> SKLQATKTLAADVIMRSPVSWKQELTLDAGRSKGASENMLAIANGGLIGSVSK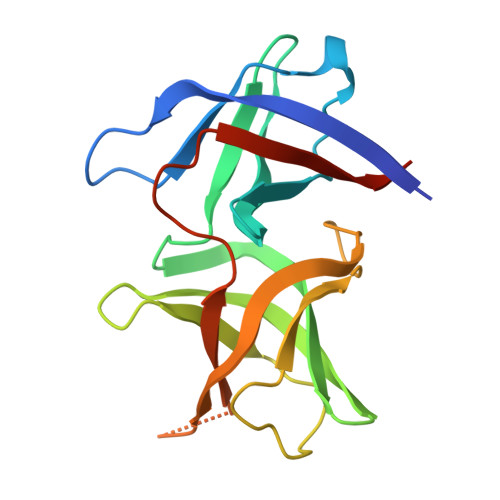VEENSTIVNLLTNTENADKISVKIQHGSTTIYGIIIGYDKENDVLKISQLNSNSDISAGDKVTTGGLGNFNVADIPVGEVVATTHSTDYLTREVTVKLSADTHNVDVIELVGNSKLVPR[4-amino-7-(propan-2-yl)-7H-pyrrolo[2,3-d]pyrimidin-5-yl](6-{[(3S,4R)-4-(4-fluorophenyl)tetrahydrofuran-3-yl]amino}pyrazin-2-yl)methanone | C24 H24 F N7 O2 | 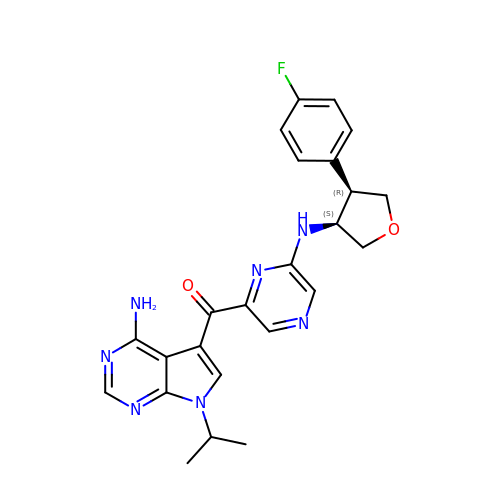YXZBQCQAYNRRFP-IEBWSBKVSA-N> MTQFEGFTNLYQVSKTLRFELIPQGKTLKHIQEQGFIEEDKARNDHYKELKPIIDRIYKTYADQCLQLVQLDWENLSAAIDSYRKEKTEETRNALIEEQATYRNAIHDYFIGRTDNLTDAINKRHAEIYKGLFKAELFNGKVLKQLGTVTTTEHENALLRSFDKFTTYFSGFYENRKNVFSAEDISTAIPHRIVQDNFPKFKENCHIFTRLITAVPSLREHFENVKKAIGIFVSTSIEEVFSFPFYNQLLTQTQIDLYNQLLGGISREAGTEKIKGLNEVLNLAIQKNDETAHIIASLPHRFIPLFKQILSDRNTLSFILEEFKSDEEVIQSFCKYKTLLRNENVLETAEALFNELNSIDLTHIFISHKKLETISSALCDHWDTLRNALYERRISELTGKITKSAKEKVQRSLKHEDINLQEIISAAGKELSEAFKQKTSEILSHAHAALDQPLPTTLKKQEEKEILKSQLDSLLGLYHLLDWFAVDESNEVDPEFSARLTGIKLEMEPSLSFYNKARNYATKKPYSVEKFKLNFQMPTLASGWDVNKEKNNGAILFVKNGLYYLGIMPKQKGRYKALSFEPTEKTSEGFDKMYYDYFPDAAKMIPKCSTQLKAVTAHFQTHTTPILLSNNFIEPLEITKEIYDLNNPEKEPKKFQTAYAKKTGDQKGYREALCKWIDFTRDFLSKYTKTTSIDLSSLRPSSQYKDLGEYYAELNPLLYHISFQRIAEKEIMDAVETGKLYLFQIYNKDFAKGHHGKPNLHTLYWTGLFSPENLAKTSIKLNGQAELFYRPKSRMKRMAHRLGEKMLNKKLKDQKTPIPDTLYQELYDYVNHRLSHDLSDEARALLPNVITKEVSHEIIKDRRFTSDKFFFHVPITLNYQAANSPSKFNQRVNAYLKEHPETPIIGIDRGERNLIYITVIDSTGKILEQRSLNTIQQFDYQKKLDNREKERVAARQAWSVVGTIKDLKQGYLSQVIHEIVDLMIHYQAVVVLENLNFGFKSKRTGIAEKAVYQQFEKMLIDKLNCLVLKDYPAEKVGGVLNPYQLTDQFTSFAKMGTQSGFLFYVPA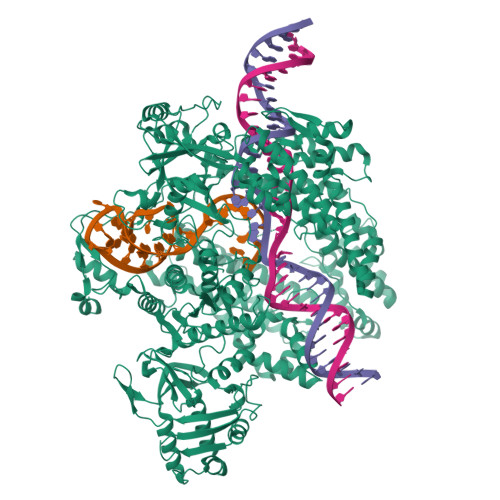PYTSKIDPLTGFVDPFVWKTIKNHESRKHFLEGFDFLHYDVKTGDFILHFKMNRNLSFQRGLPGFMPAWDIVFEKNETQFDAKGTPFIAGKRIVPVIENHRFTGRYRDLYPANELIALLEEKGIVFRDGSNILPKLLENDDSHAIDTMVALIRSVLQMRNSNAATGEDYINSPVRDLNGVCFDSRFQNPEWPMDADANGAYHIALKGQLLLNHLKESKDLKLQNGISNQDWLAYIQELRN> AYDES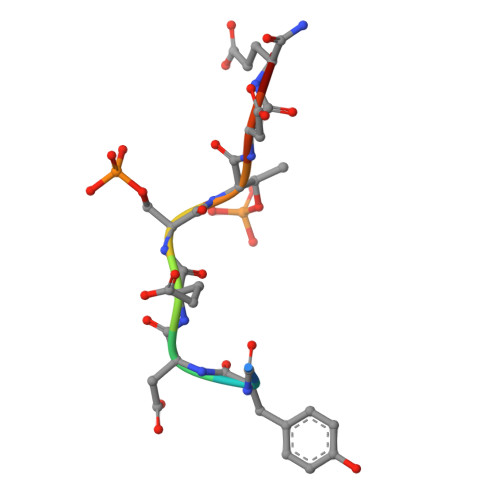TDEE> GSEVYQSQKCELKYSKSQIEKAARKIRHGCEGAEREEAIKMIQNFRELHLYPLMLMKNHLDRAAKKVDKENKIIVARRLKRLSTIIDKLERPSLDGGATNNAIALTRMQDIGGCRAIVRNIEQLKKLKDRLVKSRSKHKILKEYDYLTPKPSGYSGIHLAYSCFDEENGNNPWSKTKIEVQLRTELQHAWATSLEIIDTLENIKLKTSNEGHPEWRRFFYLSGCLVAHDEGACILDDETIKNYQTELKTLEEALSVRSKLSTYTFAMKLTSDANLKKSLPKNHNGFFLVRMRNAITKNGKDTGKFLVSVKPFRKKESEQALQELNKDDADPEVLIAVLLATNNIKSLKKAYPNYFGSTNQFGRFLSRHIDTV;> MKHHHHHHGSSGMQDQIDAKVIRRNPELTPGIFKKGIEITIDLEEMVCYHSGLTWKVKQLTNTLWSLAGDEHTVMEVI

We recently identified and characterized a fused toxin–antitoxin system called CapRelSJ46 that protects Escherichia coli against diverse phages. CapRelSJ46 contains an N-terminal toxin domain and a C-terminal antitoxin domain that normally binds and autoinhibits the N-terminal toxin. Activated CapRelSJ46 then pyrophosphorylates the 3′ end of transfer RNAs, which inhibits protein translation and restricts phage propagation. Here we discovered an additional protein trigger for CapRelSJ46 in the phage Bas11. This alternative trigger, Gp54Bas11, is a small protein of 66 amino acids with unknown function.

Next, we determined the structure of a CapRelSJ46–Gp54Bas11 complex to 2.2 Å resolution. This complex had ATP bound in the pyrophosphate donor site, stacked between R79 and R116, similar to that of other RelA/SpoT homologue enzymes, which indicated that the complex captures the active state of the enzyme. In the complex, the hydrophobic core of the Gp54Bas11 β-barrel binds to both the amphipathic anchor-1 and pseudo-ZFD of CapRelSJ46. In particular, G24, I25, S39, L41 and W43 of Gp54Bas11 contact the pseudo-ZFD β-sheet, and W53 of Gp54Bas11 becomes embedded between L270 and L276 of anchor-1 in CapRelSJ46 and I29 and L31 of Gp54Bas11. The interface is further stabilized by a polar network between D273, N275, K278 and S279 from CapRelSJ46 and Q47 and N50 from Gp54Bas11. Notably, binding of Gp54Bas11 to CapRelSJ46 involves a significant topological rearrangement. In the complex, the β-barrel of Gp54Bas11 unfolds with β1 and β6 becoming disordered, consistent with the entropy-driven binding suggested by ITC. Whereas Gp54Bas11 β2–β5 bind on one side of the pseudo-ZFD of CapRelSJ46 interacting with β7 and anchor-1, the long β1–β2 loop of Gp54Bas11 folds into β-strand β1′ and binds on the other side, making contacts with β8 of the pseudo-ZFD and effectively clamping the pseudo-ZFD. These interactions produce a ‘hybrid’ eight-stranded, antiparallel, twisted β-sheet comprising β-strands from both Gp54Bas11 and CapRelSJ46 that wraps around anchor-1 of CapRelSJ46. In addition, binding by β1′ of Gp54Bas11 to CapRelSJ46 β8 moves the pseudo-ZFD further from the active site compared with the unbound open state of CapRelSJ46, which probably primes the enzyme to bind and modify target tRNAs.> MSQPCPCGSADEYSLCCGRIVSGERVAPDPSHLMRSRYCAFVMKDADYLIKSWHPTCNAA;> AFRDDIIAGFANTRWLGLTIFEHTWSEAENTGYVSFIARFSEQGKNGAIIERSRFIKENG;> QWYYIDGTRPQLGRNDPCPCGSGKKFKKCCG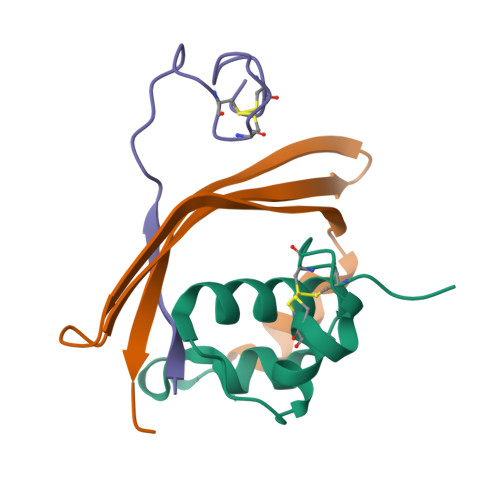Q>FKRIVQRCKD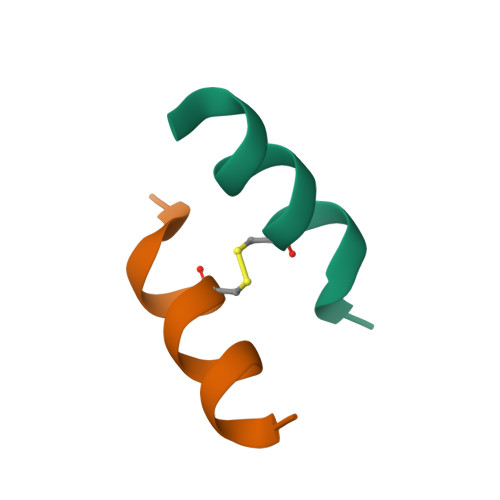FLR[2x]> MKNTPQHKLFFVVALLLVVQILAGCKSSSSTTAGSTENSSSSTPDPDTGTTTPDPIEPEVVPPVTPPSVDSNSREVIPLWEDKVADGKAWSTHVYSALD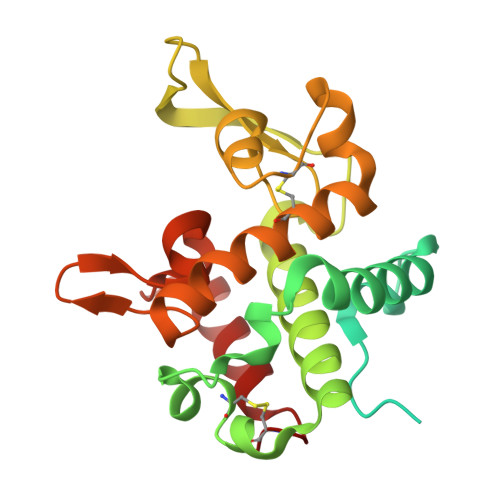KLGPNLLDVIPADRSLFCPKYSSLSYAQRKQYWAFVLSSMVRFQSNFKTAMSYTEDFNDSNGNRVISRGLLQISIESGNAYGCGFKSTKDLHDPLQNLSCGIRILDRWVSRDGRIAGKVDGAWKGGARYWSVLRAGDKTSYKSIVSWSQNLSICK> KACTRECGNLGFGICPRSEGSPLNPICINCCSGYKGCNYYNSFGKFICEGESDPKRPNACTFNCDPNIAYSRCPRSQGKSLIYPTGCTTCCTGYKGCYYFGKDG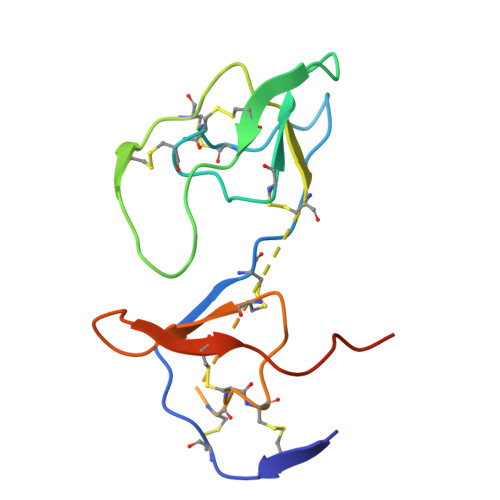KFVCEGESDEPKANMYPVM> GMQQVIKDLFYVVPLSRNCEKIYKNKTHILLGISPFNSKFSQNYIHQLIDWSSKNFKNVTVLLAGDEAKNLLEALGTPTTKAERKVRKEIRRHFRFSEEALRKNGREIDIYTFSD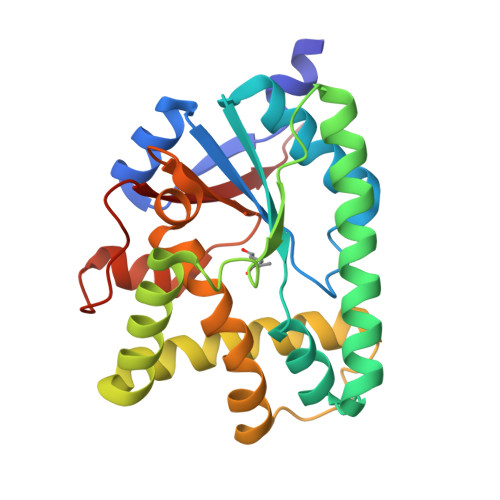FKNNKIYNEVYQNVIYYFEKDEKFRKSCLAMSHDALSSAAKSLNMEDIEITDNMLFHAVKYVLAELPFFLSGASILGYKESVLAYHRPWKLGEKIKNSEFYIKMSDNQGYIILKQIN> FV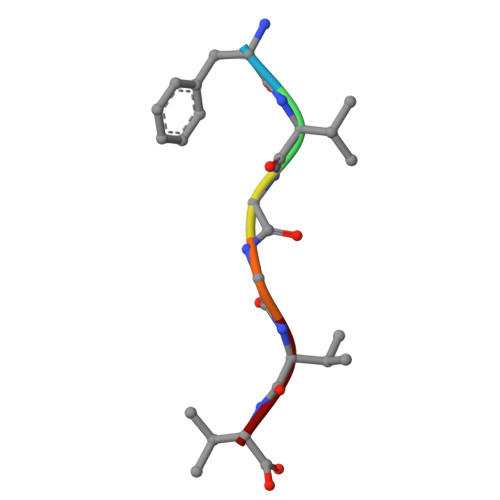GGVV(2S)-1-{[(S)-hydroxy{[(1s,2R,3R,4R,5S,6S)-2,3,4,5,6-pentahydroxycyclohexyl]oxy}phosphoryl]oxy}-3-(octadecanoyloxy)propan-2-yl 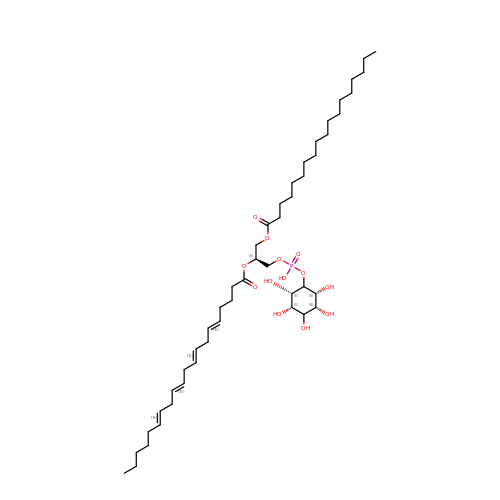(5E,8E,11E,14E)-icosa-5,8,11,14-tetraenoate | C47 H83 O13 P | KRTOMQDUKGRFDJ-ROVRCULJSA-N>[4x]MADEIA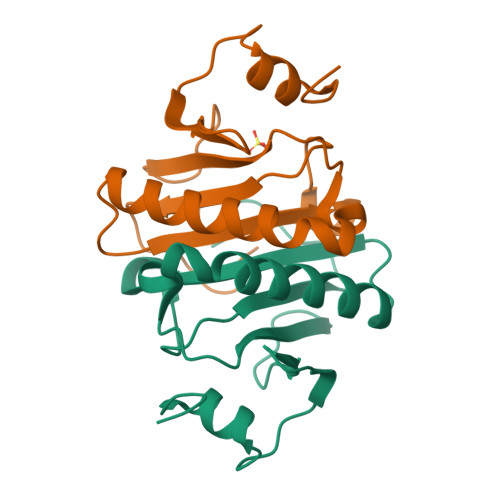KAQVARPGGDTIFGKIIRKEIPAKIIFEDDRCLAFHDISPQAPTHFLVIPKKHISQISVAEDDDESLLGHLMIVGKKCAADLGLNKGYRMVVNEGSDGGQSVYHVHLHVLGGRQMHWPPG>[6x]GPDAAVENPRIGRAADLYELIPEYQPDTYRNMDKVYPTRVIHKGTKVRPLPAGVAIAPRYRIGGEEYGVDDFMRRNRVGGVLVLKDGKVALERYGLGNDERTRWTSFSVVKSISSTLVGAAVQQGLLALDQPVDKYLPSLAGSAYQGVTVEQVLQMSSGVRWNETYRDPKSDRRQMFDAQLAERPGGILRLLASLPRQYPSGTHFTYSTGESHLQSELLHAATRIPVSDYLSERIW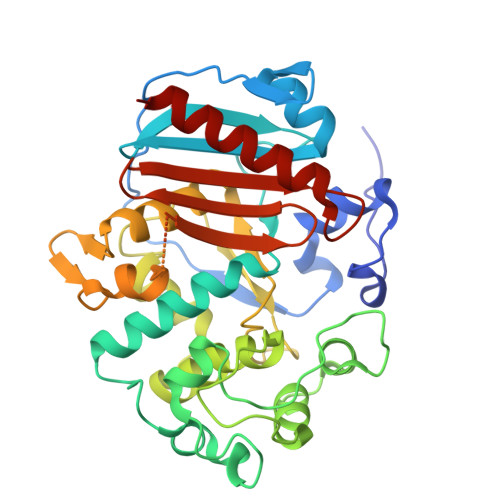ARMGMESDGFWQLESPAGQEIGSSGLSATLRDYGRFGQFVLEDGVIDGERILPEGWVDRASRVEASSHLAPGKLYDGEYALGYGYQWWTFPVGAKALPEHDGGAFEAQGIFGQYLYINRKEKIVAVVWSAWPKPEMDDREEETYAFLGAAVKALR>[2x]GEDGYIADGDNCTYICTFNNYCHALCT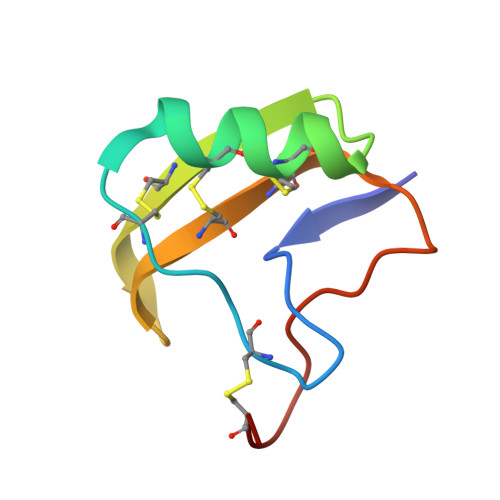DKKGDSGACDWWVPYGVVCWCEDLPTPVPIRGSGKCR> GAMGSKISEQLKCCSGILKEMFAKKHAAYAWPFYKPVDVEALGLHDYCDIIKHPMDMSTIKSKLESREYRDAQEFGADV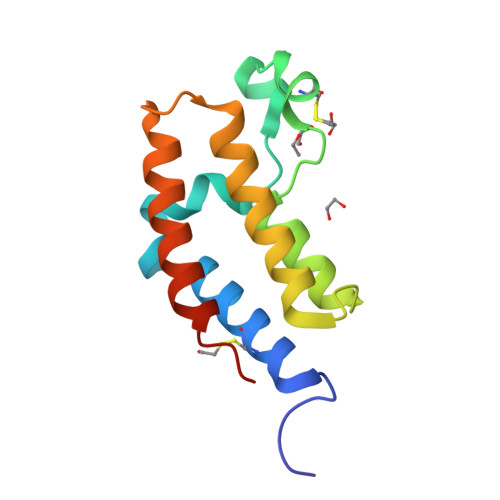RLMFSNCYKYNPPDHEVVAMARKLQDVFEMRFAKMPDEPEE>[3x]HEAGEFFMRAGSATVRPTEGAGGTLGSLGGFSVTNNTQLGLTFTYMATDNIGVELLAATPFRHKIGT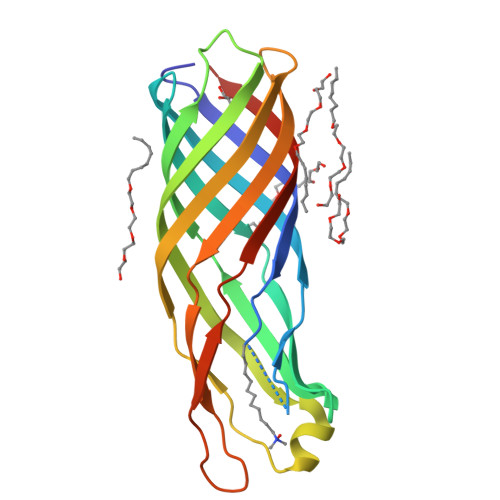RATGDIATVHHLPPTLMAQWYFGDASSKFRPYVGAGINYTTFFDNGFNDHGKEAGLSDLSLKDSWGAAGQVGVDYLINRDWLVNMSVWYMDIDTTANYKLGGAQQHDSVRLDPWVFMFSAGYRFHHHHHH> MPKRIVYNISSDFQLKSLLGEGAYGVVCSATHKPTGEIVAIKKIEPFDKPLFALRTLREIKILKHFKHENIITIFNIQRPDSFENFNEVYIIQELMQTDLHRVISTQMLSDDHIQYFIYQTLRAVKVLHGSNVIHRDLKPSNLLINSNCDLKVCDFGLARIIDESAADNSEPTGQQSGMVEFVATRWYRAPEVMLTSAKYSRAMDVWSCGCILAELFLRRPIFPGRDYRHQLLLIFGIIGTPHSDNDLRCIESPRAREYIKSLPMYPAAPLEKMFPRVNPKGIDLLQRMLVFDPAKRITAKEALEHPYLQTYHDPNDEPEGEPIPPSFFEFDHYKEALTTKDLKKLIWNEIFS;> RRNLKGLNLNLH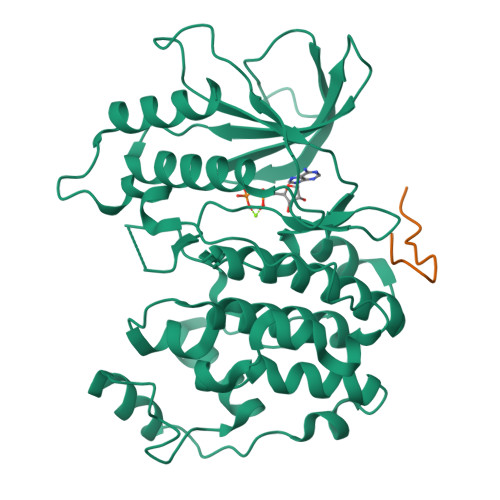PD prop-2-en-1-yl 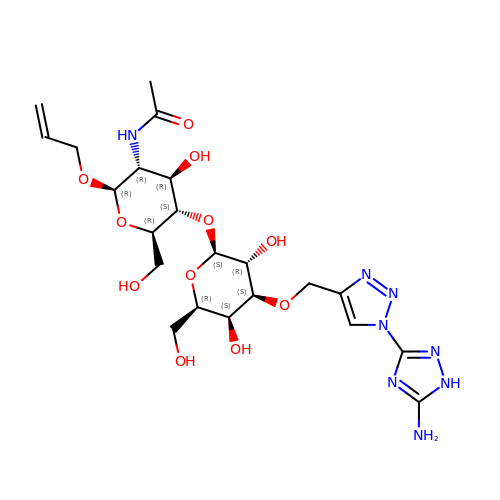2-(acetylamino)-4-O-(3-O-{[1-(5-amino-1H-1,2,4-triazol-3-yl)-1H-1,2,3-triazol-4-yl]methyl}-beta-D-galactopyranosyl)-2-deoxy-beta-D-glucopyranoside | C22 H34 N8 O11 | WCBZMORIGCDSQZ-MRHFAZSRSA-N>MQNNSYGYAVSVRVGGKEHRHWERYDIDSDFLIPADSFDFVIGRLGPEAAIPDLSGESCEVVIDGQIVMTGIIGSQRHGKSKGSRELSLSGRDLAGFLVDCSAPQLNVKGMTVLDAAKKLAAPWPQIKAVVLKAENNPALGKIDIEPGETVWQALTHIANSVGLHPWLEPDGTLVVGGADYSSPPVATLCWSRTDSRCNIERMDI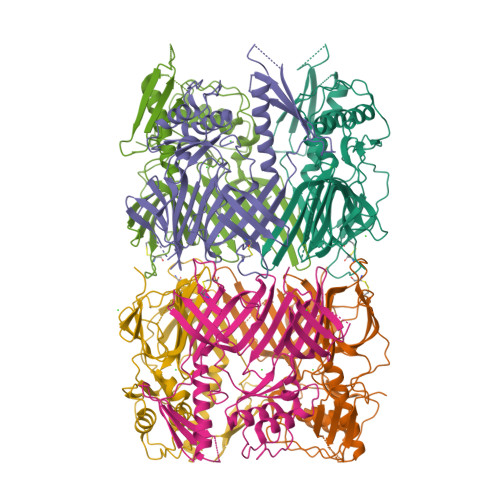EWDTDNRFSEVTFLAQSHGRSGDSAKHDLKWVYKDPTMTLHRPKTVVVSDADNLAALQKQAKKQLADWRLEGFTLTITVGGHKTRDGVLWQPGLRVHVIDDEHGIDAVFFLMGRRFMLSRMDGTQTELRLKEDGIWTPDAYPKKAEAARKRKGKRKGVSHKGKKGGKKQAETAVFE[2x]>[4x]MRGSHHHHHHGSAERMLATIMFTDIVGSTQHAAALGDDRWRDLLDNH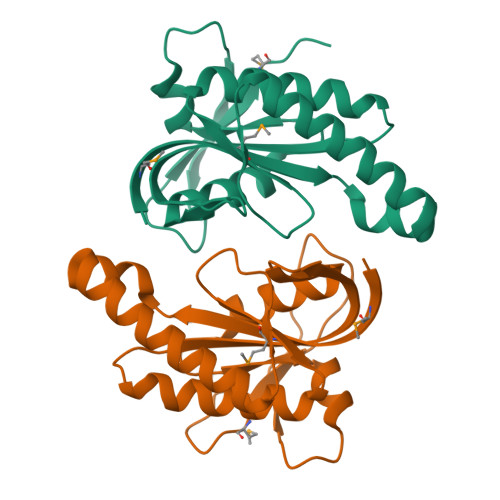DTIVCHEIQRFGGREVNTAGDGFVATFTSPSAAIACADDIVDAVAALGIEVRIGIHAGEVEVRDASHGTDVAGVAVHIGARVCALAGPSEVLVSSTVRDIVAGSRHRFAERGEQELKGVPGRWRLCVLMRDDATRTR> AQNRTIDGTDNNLSHNVWGSTNQHLDRAGPAAYADGMSMPAGGSRPSARAVSNGIAAQTGSMLNDRMLSDWVWQWGQFLDHDLDLTDAASPAESFPIPVPMGDPFFDPFNTGTQTIGLSRSAYDPATGSVDARQQMNQITSWIDASNVYGSDMTRANALRTMSGGRLATSAGDLLPFNTGGLPNAGGTSPSLFLAGDVRSNEQSGLAAVHTLFVREHNRLADQIAAANPGMGDEDIYQQARKIVGAQMQIITYNEFLPALLGSAAPSPMSIGYDDSINPNIMNEFANACYRVGHTMLSPTILRLDNAGNVIPHGNLALQDAFFNPNRIINEGGIAPILKGLASQAMQEIDNKIVDDVRNFLFGPPGSGGLDLASLNIQRGRDHGLPDYNSTRVMMGLTSVSSFADISSDPAVQAALMSLYGTVNDIDLWVGALAEDHLAGSSVGELIAAVLGEQFTRLRDGDRYWYERDDFFVNNPSLLAELQATRLSDIIRRNSDITNIQDNVFLIPEPATLGLLMFGAAFLRKRRS

Although CyanoPOX shares relatively low sequence identity (37 %) with bovine lactoperoxidase, it displays comparable biochemical properties. Except for a highly similar overall structure, CyanoPOX also has a conserved active site pocket when compared with mammalian lactoperoxidases.

The crystal structure of CyanoPOX with a bound heme cofactor was determined at 1.67 Å resolution in the monoclinic space group P21 with one molecule in the asymmetric unit. Also, CyanoPOX in the crystal structure seems monomeric, with a size of 55×50×44 Å. Unlike eukaryotic peroxidases, CyanoPOX lacks disulfide bridges and N‐glycosylation sites. A non‐covalently bound b‐type heme cofactor is situated in the central core of the CyanoPOX structure. On the proximal heme site the conserved residues, His294, Leu372, Asn376 and Arg291 are situated. His81 is identified as the distal heme ligand. One of the propionate chains of the heme has salt bridges with the side chains of Arg291 and Arg379. The covalent bonds with the methyl groups of the heme observed in mammalian peroxidases to Asp80 and Glu202 (CyanoPOX numbering), through two ester bonds between OD2‐Asp and heme atom CMD, and OE2‐Glu and heme atom CMB, are absent, but the residues nevertheless remain. A conserved calcium ion is observed on the distal site of the heme (11 Å to His81). Another non‐conserved calcium ion (10 Å to His294) is liganded by the sidechain of Asp350, the carbonyl oxygen and OG1 of Thr295 (adjacent to His294), the carbonyl oxygens of Glu348 and Lys352, and two water molecules.>MHHHHHHMGDALGLIETKGLVACIEAADAMCAAANVELIGYGNVGSGLVTAMVKGDVGAVK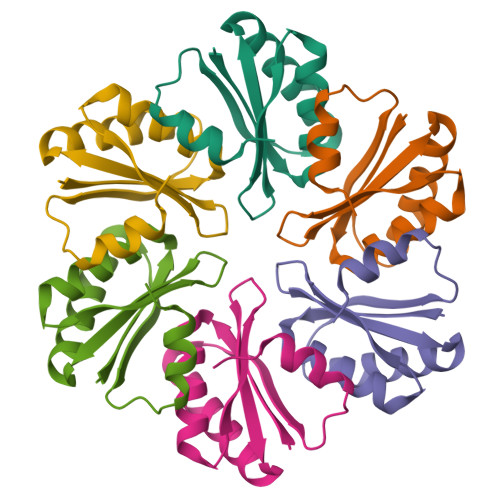AAVDSGVESAQRIGEVVTSLVIARPHNDINKIVSHYKITD[6x]>[2x]HHHHHHFNLPPGNYKKPKLLYCSNGGHFLRILPDGTVDGTRDRSDQHIQLQLSAESVGEVYIKSTETGQYLAMDTDGLLYGSQTPNEECLFLE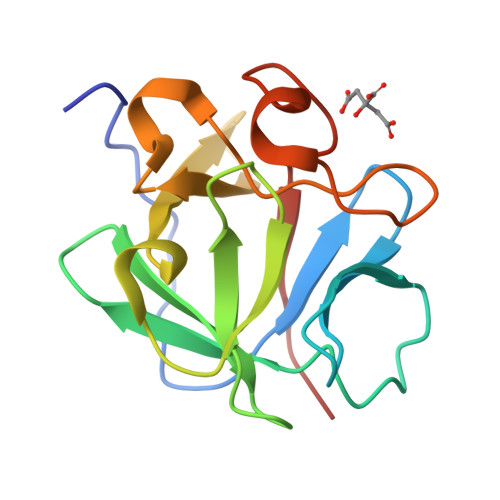RLEENHYNTYISKKHAEKNWFVGLKKNGSAKRGPRTHYGQKAILFLPLPVSSD> MLLNPTKRERKENYSIDNYYKDVLNTGRSSTPSHPRMPKPHVFHSHQLQPPQLKVLYEKERMWTAKKTGY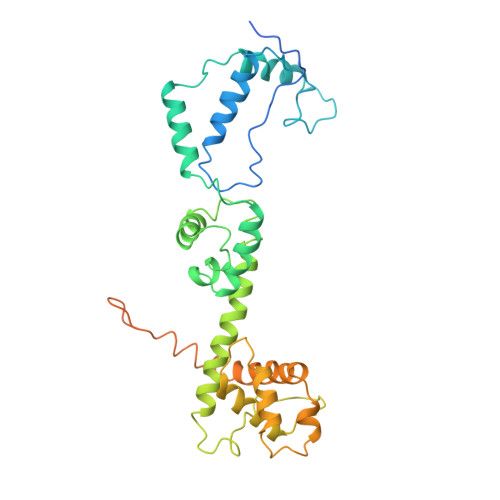VPTMDDVKAAYGDISDEEEKKQKLELLKLSVNNSQPLTEEEEKMKADWESEGFTNWNKLEFRKFITVSGKYGRNSIQAIARELAPGKTLEEVRAYAKAFWSNIERIEDYEKYLKIIENEEEKIKRVKMQQEALRRKLSEYKNPFFDLKLKHPPSSNNKRTYSEEEDRFILLMLFKYGLDRDDVYELVRDEIRDCPLFELDFYFRSRTPVELARRGNTLLQCLEKEFNAGIVLDDATKDRMKKEDENGKRIREEFADQTANEKENVDGVESKKAKIEDTSNVGTEQLVAEKIPENETTHHHHHHH>GNMEASEVMKEKGNAAYKGKQWNKAVNFYTEAIKLNGANATYYCNRAAAFLELCCFQQAEQDCTKAMLIDKKNVKAYLRRGTAREELVRYKEAAADFRHALVLEPQNKTAKVAEKRLRKHI[2x];>GSKMEEVD[2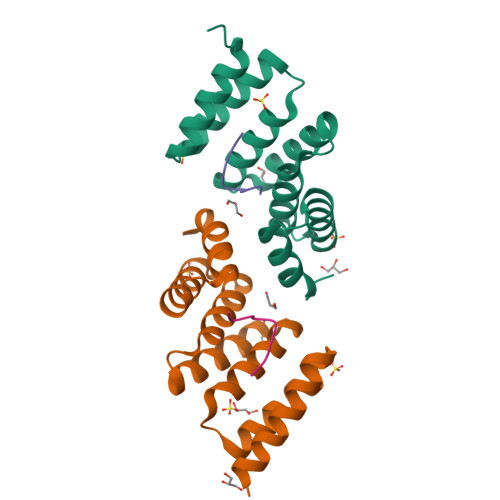x]> GSPGIL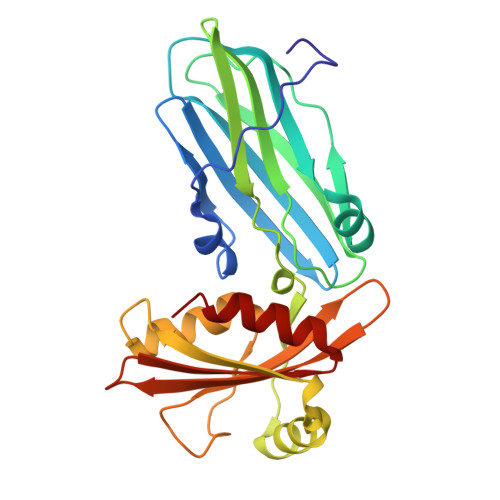APLAPGSEDNFARFVCKNNGVLFENQLLQIGLKSEFRQNLGRMFIFYGNKTSTQFLNFTPTLICADDLQTNLNLQTKPVKPTVDGGAQVQQVVNIECISDFTEAPVLNIQFRYGGTFQNVSVKLPITLNKFFQPTEMASQDFFQRWKQLSNPQQEVQNIFKAKHPMDTEITKAKIIGFGSALLEEVDPNPANFVGAGIIHTKTTQIGCLLRLEPNLQAQMYRLTLRTSKDTVSQRLCELLSEQF> MAQAFVDATWPQAAKAAQSLGVPAHFLVAQAALETGWGKSQIRNKDGTPSYNLFNIKAGSNWTGKVVEARTVEYENGQRKVRVERFRAYDSYEQAFQDYADLVGNSPRYAKVAGKTDGHAFARALQEGGYATDPSYADKLARVINGNALRQRLMA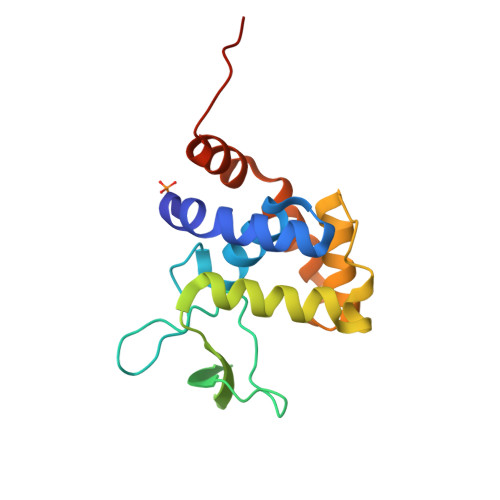SAASARGLEHHHHHH> QISVRGLAGVENVTELKKNFNRHLHFTLVKDRNVATPRDYYFALAHTVRDHLVGRWIRTQQHYYEKDPKRIYYLSLEFYMGRTLQNTMVNLALENACDEATYQLGLDMEELEEIEEDAGLGNGGLGRLAACFLDSMATLGLAAYGYGIRYEFGIFNQKICGGWQMEEADDWLRYGNPWEKARPEFTLPVHFYGRVEHTSQGAKWVDTQVVLAMPYDTPVPGYRNNVVNTMRLWSAKAPNDFNLKDFNVGGYIQAVLDRNLAENISRVLYPNDNFFEGKELRLKQEYFVVAATLQDIIRRFKSSKFGCRDPVRTNFDAFPDKVAIQLNDTHPSLAIPELMRVLVDLERLDWDKAWEVTVKTCAYTNHTVLPEALERWPVHLLETLLPRHLQIIYEINQRFLNRVAAAFPGDVDRLRRMSLVEEGAVKRINMAHLCIAGSHAVNGVARIHSEILKKTIFKDFYELEPHKFQNKTNGITPRRWLVLCNPGLAEIIAERIGEEYISDLDQLRKLLSYVDDEAFIRDVAKVKQENKLKFAAYLEREYKVHINPNSLFDVQVKRIHEYKRQLLNCLHVITLYNRIKKEPNKFVVPRTVMIGGKAAPGYHMAKMIIKLITAIGDVVNHDPVVGDRLRVIFLENYRVSLAEKVIPAADL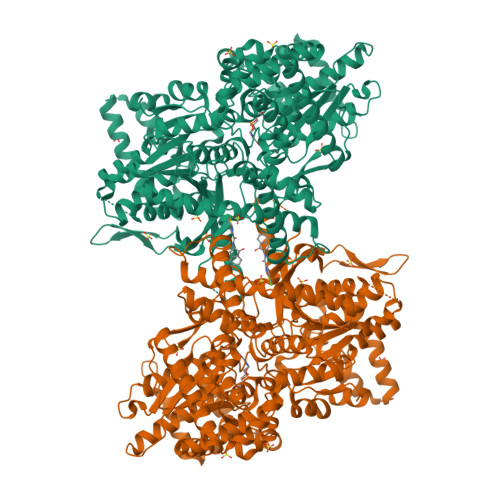SEQISTAGTEASGTGNMKFMLNGALTIGTMDGANVEMAEEAGEENFFIFGMRVEDVDRLDQRGYNAQEYYDRIPELRQIIEQLSSGFFSPKQPDLFKDIVNMLMHHDRFKVFADYEEYVKCQERVSALYKNPREWTRMVIRNIATSGKFSSDRTIAQYAREIWGVEPSRQRLP> LVPRGSHMSIFDKRVNYKPFEYPEVLQFTEAINKAYWVHTEVDFTADTQDFHAHLSLAEKTAVKNSLLAI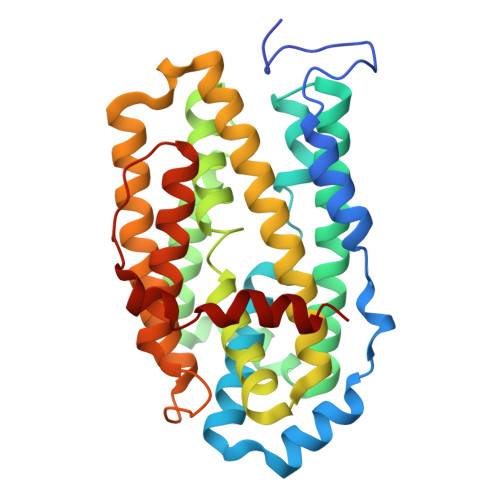AQIEVAVKSFWGNIYEHFPKPEFNGLGSTFAECEFRHSEAYSRLLEVLGYNDEFEKLLDVPVIRRRVDYLSNVLKDTKSQDNRKYMVSLILFSILIENVSLFSQFAILLSFTRFKGYMKNVSNIIAWTSIDEQIHANGGIYIINKIREEFPDYFDEETLALVRETVKDSIAVESDILDWIFEEGEIESIKKGDLVNFMKFRIDESLKQINIPVIFDVKVEDYKALAWFEEEVFANSL1-[GLYCEROLYLPHOSPHONYL]-2-[8-(2-HEXYL-CYCLOPROPYL)-OCTANAL-1-YL]-3-[HEXADECANAL-1-YL]-GLYCEROL | C39 H75 O10 P | 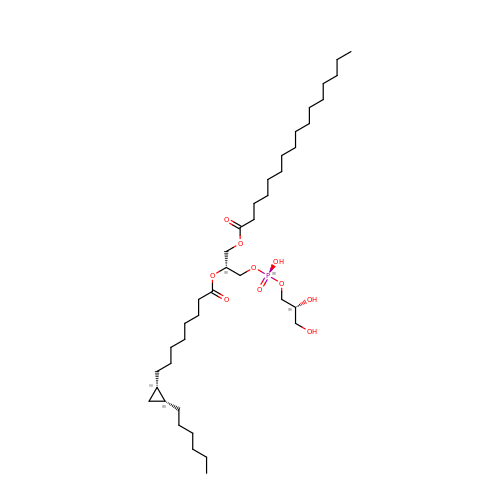JWIOKCJPLNKYBQ-JIZALCTLSA-N> MIHCLRNIRTVSALQSKISYNLGGGNKRKKTSGDLDNYDVLFVGANLGGICSNHFDKDTHGKYKCFVSFDQPINQIYSVRIPYEQQRVRKSEYIHFSKKSINQFTPSEMLAVKEILPEQNAVVLSSGRRIGYNQLVLATGLKHDFSQIKGFYEALEHPEHPVYANRDPETWRSAQHKYSKYISNFKSGDGYFCIPEYPYAGEVECFNFFVSDEVWKWAQHHGALSPKHTFTIVNANEKFVHYCDSADAFIKERLEKRGIRVEY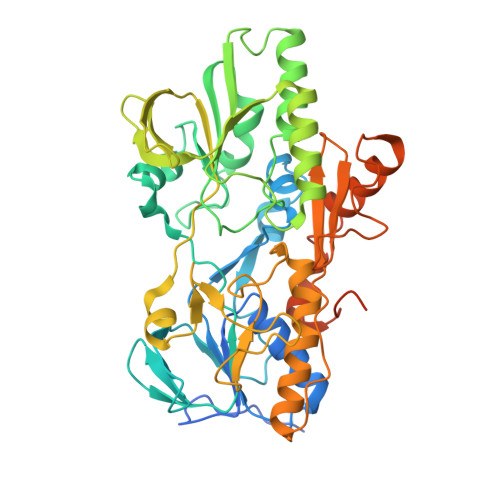NTKLLEVHQDGQKATFINTKTGEKSVRDYNNLYSIVPSKRQEFLDKAGLTNGNGLLNVDHQTLQHKKYKNIFGLGDAADLPTTKTFWAGWYQIAVVRNNVKRNLQGQTLNAHYDGFSKVPLFTGHQTLTYVAHSYGGVGNWQHLKHNNGGILAWMRYRSWAKGMAKKFQDFYNGARLGPPYHKVLKSFPELPGSPESQQSSGISKYFPTKTENKAAH> NLIPTVIEQTNRGERAYDIY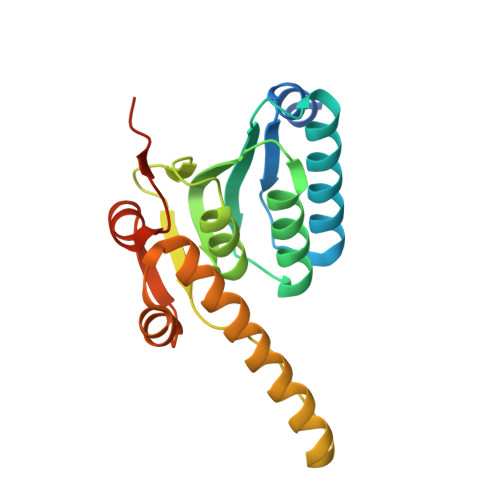SRLLKDRIIMLGSAIDDNVANSIVSQLLFLAAEDPEKEISLYINSPGGSITAGMAIYDTMQFIKPKVSTICIGMAASMGAFLLAAGEKGKRYALPNSEVMIHQPLGGAQGQATEIEIAAKRILLLRDKLNKVLAERTGQPLEVIERDTDRDNFKSAEEALEYGLIDKILTHTEDKKHHH> MGHHHHHHIFPKQYPIINFTTAGATVQSYTNF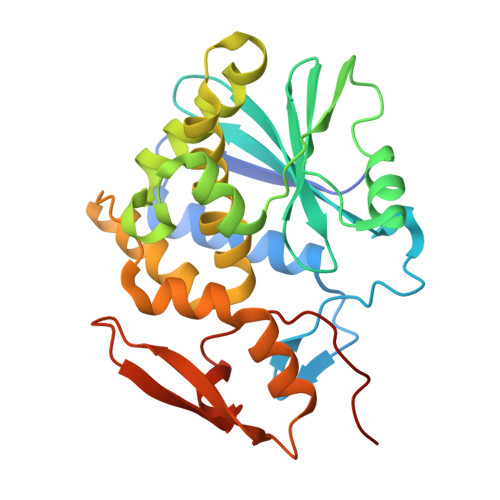IRAVRGRLTTGADVRHEIPVLPNRVGLPINQRFILVELSNHAELSVTLALDVTNAYVVGYRAGNSAYFFHPDNQEDAEAITHLFTDVQNRYTFAFGGNYDRLEQLAGNLRENIELGNGPLEEAISALYYYSTGGTQLPTLARSFIICIQMISEAARFQYIEGEMRTRIRYNRRSAPDPSVITLENSWGRLSTAIQESNQGAFASPIQLQRRNGSKFSVYDVSILIPIIALMVYRCAPPPSSQF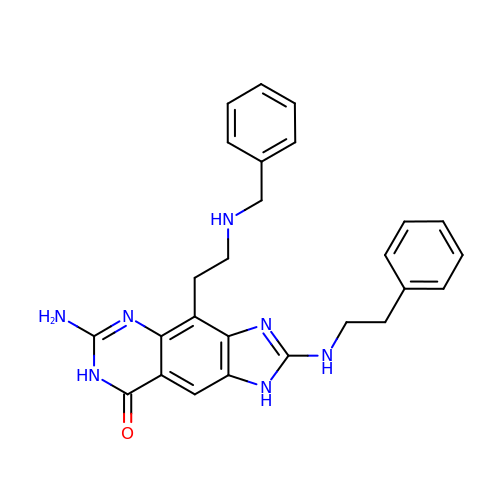6-amino-4-[2-(benzylamino)ethyl]-2-[(2-phenylethyl)amino]-1,7-dihydro-8H-imidazo[4,5-g]quinazolin-8-one | C26 H27 N7 O | YCQZLEKKVPSANH-UHFFFAOYSA-N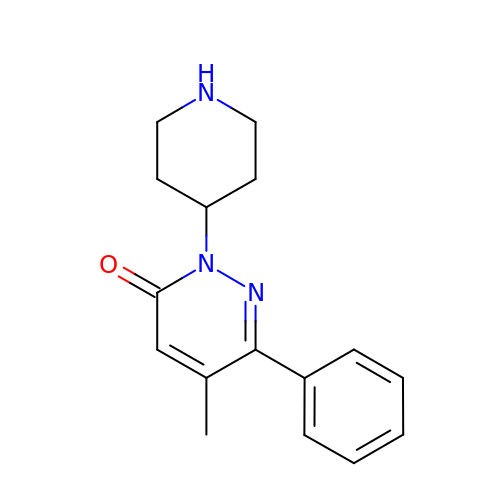5-methyl-6-phenyl-2-piperidin-4-yl-pyridazin-3-one | C16 H19 N3 O | TWZULJZXADJJPI-UHFFFAOYSA-N> SMSSFEGQMAEYPTISIDRFDRENLRARAYFLSHCHKDHMKGLRAPTLKRRLECSLKVYLYCSPVTKELLLTSPKYRFWKKRIISIEIETPTQISLVDEASGEKEEIVVTLLPAGHCPGSVMFLFQGNNGTVLYTGDFRLAQGEAARMELLHSGGRVKDIQSVYLDTTFCDPRFYQIPSREECLSGVLELVRSWITRSPYHVVWLNCKAAYGYEYLFTNLSEELGVQVHVNKLDMFRNMPEILHHLTTDRNTQIHACRHPKAEEYFQWSKLPCGITSRNRIPLHIISIKPSTMWFGERSRKTNVIVRTGESSYRACFSFHSSYSEIKDFLSYLCPVNAYP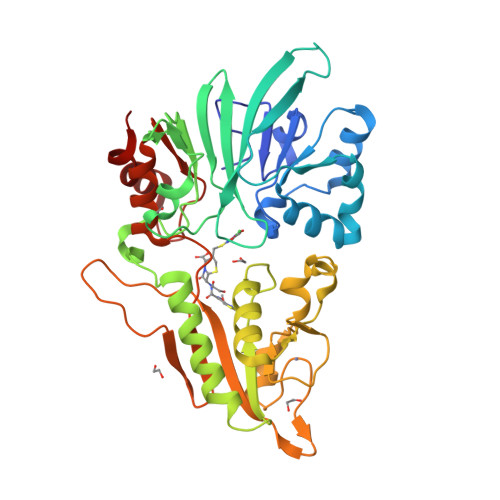NVIPVGTTMDKVVEILKPLCRS PIMELIC ACID | C7 H12 O4 | 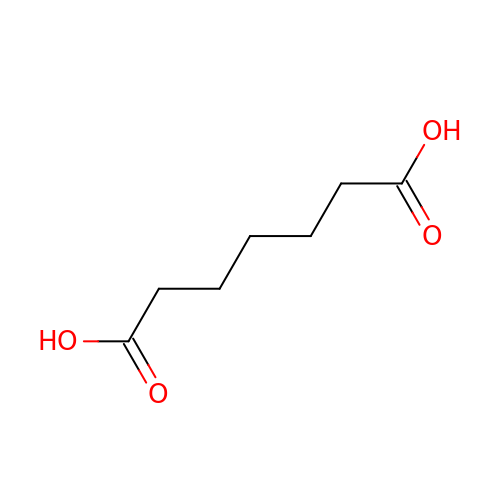WLJVNTCWHIRURA-UHFFFAOYSA-N> MAPKRSRRSNRRAGSRAAATSLVYDTCYVTLTERATTSFQRQSFPTLKGMGDRAFQVVAFTIQGVSAAPLMYNARLYNPGDTDSVHATGVQLMGTVPRTVRLTPRVGQNNWFFGNTEEAETILAIDGLVS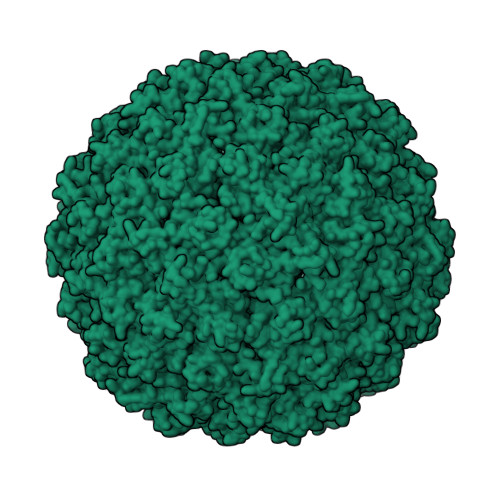TKGANAPSNTVIVTGCFRLAPSELQSS>[4x]MSGMEKFKEQLLEEVKKIVLETMTKVMEHLEKWFVTLAEIIITKSEEKLEELKETMEKSIEELRKEAEGS

Here we use deep network hallucination to generate a wide range of symmetric protein homo-oligomers given only a specification of the number of protomers and the protomer length. Starting from only a choice of chain length L and oligomer valency N (2 for a dimer, 3 for a trimer, etc.), the method carries out a Monte Carlo search in sequence space starting from a random sequence. The loss function guiding the search is computed by inputting N copies of the sequence into the AlphaFold2 (AF2) network, and combining structure prediction confidence metrics (pLDDT; per-residue structural accuracy, and pTM; an estimate of the TM-score) with a measure of cyclic symmetry (the standard deviation of the distances between the center of mass of adjacent protomers within the predicted structure). To eliminate such over-fitting, we generated new sequences for the HAL backbones using the recently developed ProteinMPNN sequence design neural network (accompanying manuscript: Dauparas et al.).

To evaluate design accuracy we attempted crystallization of 19 designs and succeeded in solving crystal structures for seven (three C2s, two C3s and two C4s). All crystal structures had the correct oligomerization state and closely matched the design models (median Cα RMSD of 0.6 Å across all designs, with resolutions ranging from 1.8 to 3.4 Å). The side chain conformations in the crystal structures also closely match those of the design models. HALC4_135 is a coiled-coil composed of helical hairpins reminiscent of HALC3_104, but with C4 symmetry instead of C3, and a discontinuous superhelical twist. Despite its simple topology, the closest structural homologue to this design has a TM-score of only 0.59.> MNQKIAEEKRKRDEINMVKDAIKLTSDFYRTIYDEFGKQASELAKELASVSQGKQIKSVDDALNAFDKFRNNLNKKYNIQDRMAISKALEAINQVHMAENFKLFSKAFGFTGKVIDRYDVAVELQKAVKTDNWRPFFVKLESLAAGRAASAVTAWAFSVMLGTPVGILGFA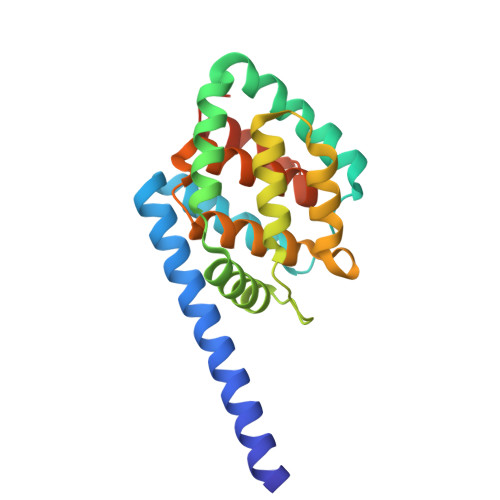IIMAAVSALVNDKFIEQVNKLIGIGSRSHHHHHH> KMLEEIMKYEASILTHDSSIRY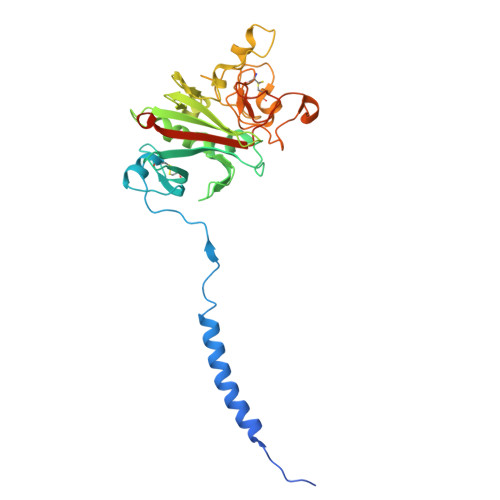LQEIYNSNNQKIVNLKEKVAQLEAQCQEPCKDTVQIHDITGKDCQDIANKGAKQSGLYFIKPLKANQQFLVYCEIDGSGNGWTVFQKRLDGSVDFKKNWIQYKEGFGHLSPTGTTEFWLGNEKIHLISTQSAIPYALRVELEDWNGRTSTADYAMFKVGPEADKYRLTYAYFAGGDAGDAFDGFDFGDDPSDKFFTSHNGMQFSTWDNDNDKFEGNCAEQDGSGWWMNKCHAGHLNGVYYQGGTYSKASTPNGYDNGIIWATWKTRWYSMKKTTMKIIPFNRLTIGEGQQHHLGGAK> AMAPAKKSEELVAEAHNLCTLLENAIQDTVREQGNSMMNLDW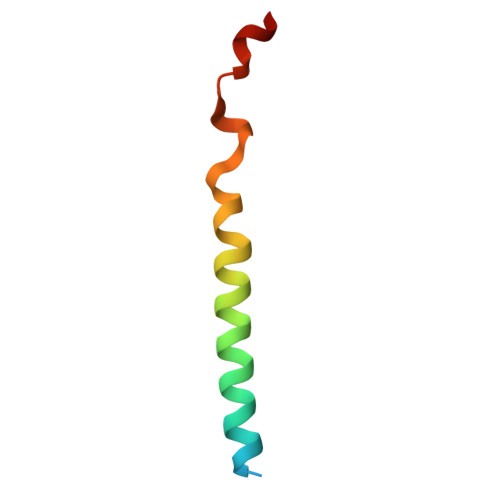SWLTE>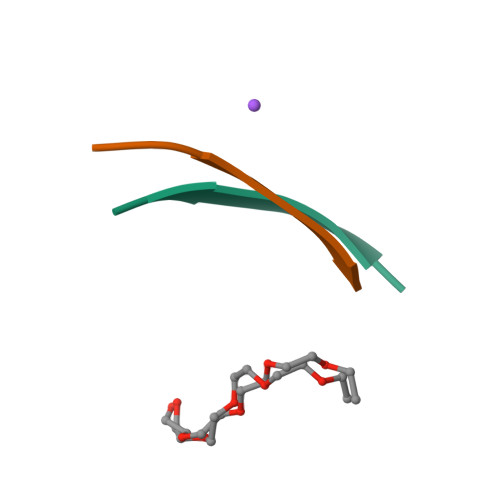[4x]KDWSFY The anti-apoptotic (pro-survival) proteins of the BCL-2 family include BCL-2, BCL-XL, MCL-1, BCL-w and BFL-1/A1. These proteins bind to and sequester the apoptosis effectors, as well as the apoptosis sensitizers, BIM, BID, PUMA, NOXA, BAD, BMF, HRK and BIK5,6. An elongated hydrophobic groove is thus formed along the surface of BCL-2 and BCL-XL proteins, spanning approximately 20 Å to serve as the binding site for the amphipathic α-helical BH3 domains of their pro-apoptotic partners. Herein we present cyclic peptides (CPs) with nanomolar-level binding affinities to BCL-2 or BCL-XL, and further reveal the structural and functional mechanisms of how these CPs target two proteins in a fashion that is remarkably different from traditional small-molecule inhibitors.

Therefore, we measured the binding affinities of cp1 to both BCL-2 and BCL-XL using a SPR assay. The results indicate that cp1 has a much higher binding affinity to BCL-2 (0.65 ± 0.14 μM) than to BCL-XL (>12 μM), implying an over 19-fold selectivity of cp1 for these two highly similar BCL-2 family proteins. To understand the beneath structural basis for this selectivity of cp1, we co-crystalized and determined the complex structures of cp1 bound to BCL-2 and BCL-XL proteins with high resolutions at 2.1 Å and 2.0 Å, respectively. In both structures, the electron densities for cp1 were well defined. Two residues of cp1 (i.e. cp1-Y5 and cp1-W7) are buried in the hydrophobic pocket formed by F104, Y108, F112, M115, L137, F138 and A149 of BCL-2 (F97, Y101, F105, L108, L130, F131 and A142 of BCL-XL). The cp1-R4 forms hydrogen bonds with E136 and L137 of BCL-2 (E129 and L130 of BCL-XL), and cp1-D8 forms a salt bridge with R146 of BCL-2 (R139 of BCL-XL), a conserved arginine residue of the pro-survival proteins known to interact with a conserved aspartate residue of the BH3-only proteins. It is noteworthy that the main-chain N atom of cp1-G6 forms a hydrogen bond with the carboxyl group of D111 in BCL-2. Therefore, we speculate that the D111/A104 discrepancy between BCL-2 and BCL-XL may be mainly responsible for the selectivity of cp1, while the M115/L108 pair is perhaps not as crucial as the former one. To test the essentiality of D111, we generated a BCL-2 D111A mutant and measured its binding affinity to cp1 also using SPR. This mutant showed a clearly lower cp1-binding affinity (5.34 ± 1.00 µM) than wild-type (WT) BCL-2 (0.65 ± 0.14 μM), yet comparable to BCL-XL (>12 µM).

> MAHAGRTGYDNREIVMKYIHYKLSQRGYEWDAGDDVEENRTEAPEGTESEVVHLTLRQAGDDFERRYRRDFAEMSSQLHLTPFTARGRFATVVEELFRDGVNWGRIVAFFEFGGVMCVESVNREMSPLVDNIALWMTEYLNRHLHTWIQDNGGWDVFVELYGPSMR;> CPARYGWDYECX>[2x]S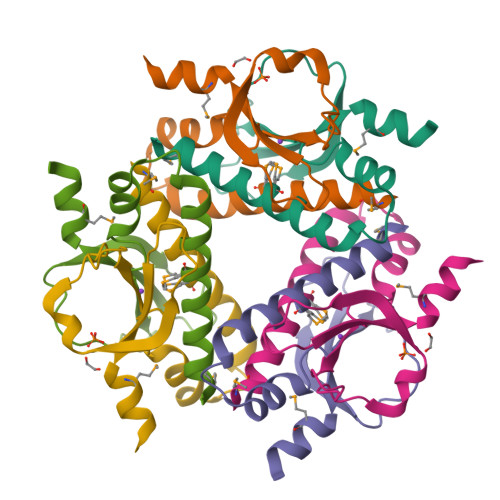NANGYTMQRDNQKTLAVYMFEEINRDVEYLSGRLSEKELKDKYRYYGRGYVRITDKDGQVITYEDGSVQDKTVFLTNEGANKLGWKLEFLIDEKMFEEEILEKQN2-(trimethylsilyl)ethyl 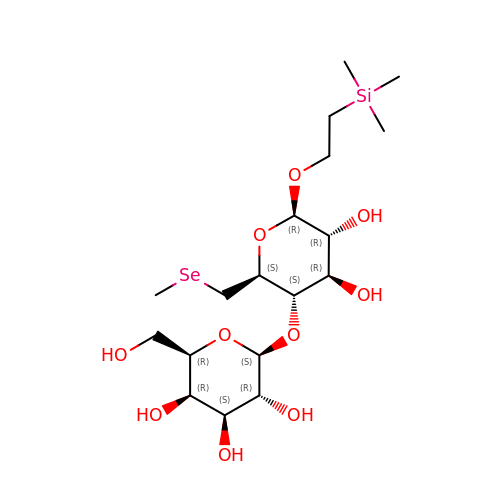4-O-beta-D-galactopyranosyl-6-Se-methyl-6-seleno-beta-D-glucopyranoside | C18 H36 O10 Se Si | DAHDBHYUNUXOAL-MUKCROHVSA-N> MVVEGVKTDFGPPYFRDLLHPVIAKNYGKWKYHEVVKPGVIKRVAESGDVIYVVRFGTPRLLSIYTVRELCDIADKYSDGYLRWTSRNNVEFFVTDESKIDDLINEVQERVGFPCGGTWDAVKGEYGLSNIVHTQGWIHCHTPAIDASGIVKAVMDELYEYFTDHKLPAMCRISLACCANMCGAVHASDIAIVGIHRTPPIPNDEAIRKTCEIPSTVAACPTGALKPDMKNKTIKVDVEKCMYCGNCYTMCPGMPLFDPENDGAAIMVGGKLSEARRMPELSKVVVPWVPNEPPRWPTLVKYVKQILEAWAANANKHERLIEWVDRIG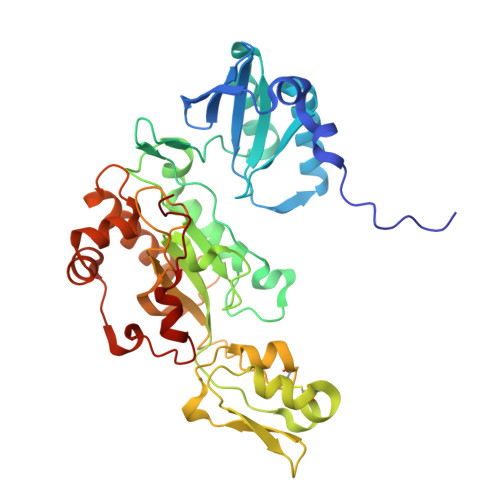WERFFELTGLEFTQHLIDDYRITPYFYSEFRASTQFKW>SHAGANDLCQECEDIVHLLTKMTKEDAFQEAIRKFLEQECDILPLKLLVPRCRQVLDVALPLVIDYFQSQINPKAICNAVGLCPRGQ[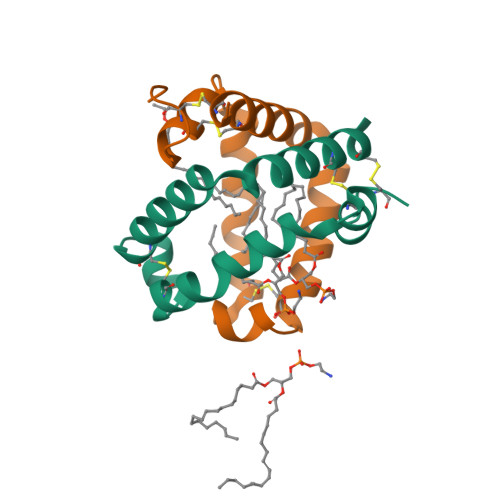8x]>[2x]MIIYRDLISHDEMFSDIYKIREIADGLCLEVEGKMVSRTEGNIDDSLIGGNASAEGPEGEGTESTVITGVDIVMNHHLQETSFTKEAYKKYIKDYMKSIKGKLEEQRPERVKPFMTGAAEQIKHILANFKNYQFFIGENMNPDGMVALLDYREDGVTPYMIFFKDGLEMEKCLEHHHHHH

Histamine-Releasing Factor (HRF), also referred to as Translationally Controlled Tumour Protein (TCTP), p21, p23 and fortilin, is ubiquitously expressed in eukaryotes, and involved in apoptosis, cell cycle progression, cell proliferation and cancer (Bommer and Thiele, 2004, Nagano-Ito and Ichikawa, 2012, Bommer, 2012). In addition to its diverse range of intracellular roles, HRF is also able to activate mast cells and basophils, with the release of histamine (MacDonald et al., 1995, Kashiwakura et al., 2012), implicating a role in allergic disease. HRF can form dimers (Yoon et al., 2000; Kim et al., 2009, Kashiwakura et al., 2012), and a disulphide-linked dimer was shown to be crucial for the cytokine-like activity of rat HRF. mHRF, hHRF and rat HRF contain two cysteine residues, at positions 28 and 172, and Cys172 is suggested to be the site of the intermolecular disulphide bond. The current model for the activity of HRF in mast cell activation involves cross-linking of FcεRI-bound IgE by dimeric HRF, mediated by interactions between HRF and the Fab regions of IgE.

The structure of hHRF-1, solved at 1.75 Å resolution, contains two molecules in the asymmetric unit. Residues 1–41 and 62–180, and 1–40 and 64–180 were modeled for chains A and B of the hHRF-1 structure, respectively, and as in the mHRF structure, a substantial portion of the mobile loop region was disordered.Fig. 2 hHRF-1. The two molecules of the asymmetric unit form non-covalent interactions, and are arranged such that their interface buries a surface area of ∼530 Å2. This particular packing arrangement is very different to that of mHRF, and has not been observed in any other HRF crystal structure. One hHRF structure, and the mHRF structure, contain non-covalent HRF interactions, but reveal different packing arrangements.>MTMQIKIKYLDETQTRISKIEQGDWIDLRAAEDVTIKKDEFKLVPLGVAMELPEGYEAHVVPRSSTYKNFGVIQTNSMGVIDESYKGDNDFWFFPAYALRDTEIKKGDRICQF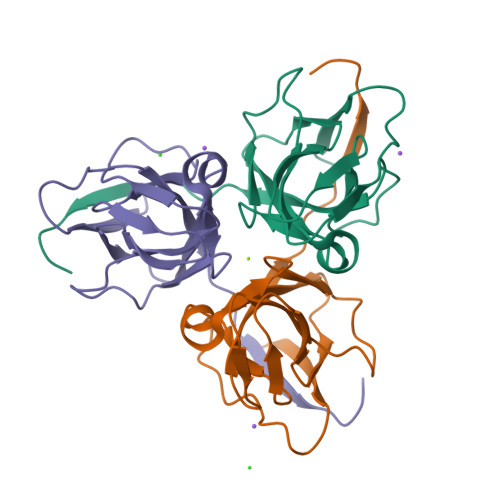RIMKKMPAVELVEVEHLGNEDRGGLGSTGTK[6x]>[3x]ATGDFPNKPLDIIVTFPPGGGTDMLARLIGNYLTESLGQTAVVENRPGASGNVGARLVADRAPDGYSLLMVNSSFAVNPGVFRNLPFDPKKDFAAVINVAYVPSVFVVPAGSKYKTLGELMAAAKQTNTQVTYGSCGNGTPQHLAGELLNVSAKTHMVHVPYKGCGPALNDVLGSQIGLAVVTASSAIPFIKAGKLQALAVTSKERSALLPEVPTVAEQGVAGYELNQWHGLLVPGATPMAVRQKL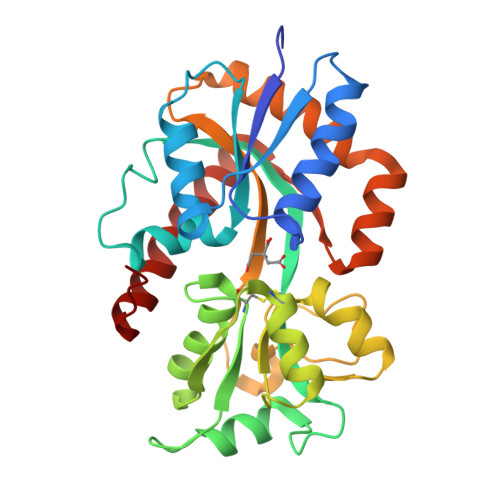YDGIAKVMQRDDVQKKLADLGYSTASDGPEVFQKMVETDIDRFSALTKQIGLKVD>AFSSF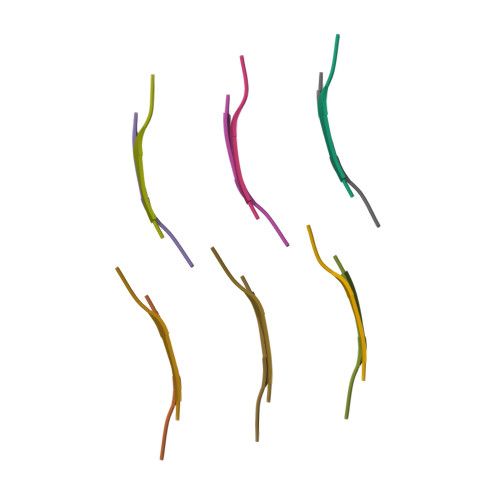N[12x]>[7x]MASMTGGQQMGTNQGKGVVAAGDKLALFLKVFGGEVLTAFARTSVTTSRHMVRSISSGKSAQFPVLGRTQAAYLAPGENLDDKRKDIKHTEKVITIDGLLTADVLIYDIEDAMNHYDVRSEYTSQLGESLAMAADGAVLAEIAGLCNVESKYNENIEGLGTATVIETTQNKAALTDQVALGKEIIAALTKARAALTKNYVPAADRVFYCDPDSYSAILAALMPNAANYAALIDPEKGSIRNVMGF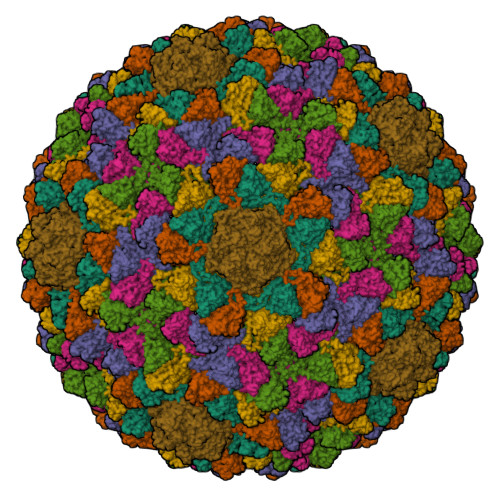EVVEVPHLTAGGAGTAREGTTGQKHVFPANKGEGNVKVAKDNVIGLFMHRSAVGTVKLRDLALERARRANFQADQIIAKYAMGHGGLRPEAAGAVVFKVE> EFSPAAAPPTLPPYFMKGSMIQLANGELKKVEDLKTEDFIQSAEMSNDLKIDSSTVERIEDSHSPGVAVIQFAVGEHRAQVSVEVLVEYPFFVFGQGWSSCCPERTSQLFD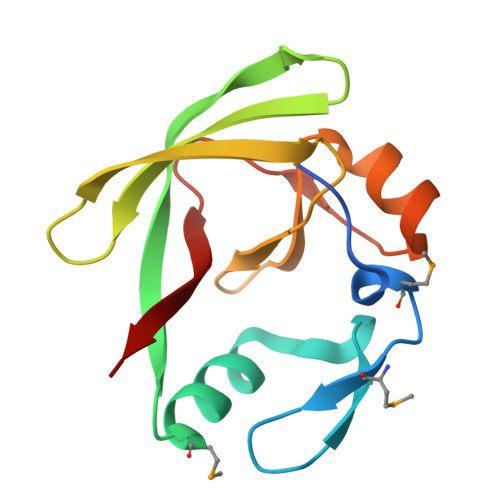LPCSKLSVGDVCISLTLK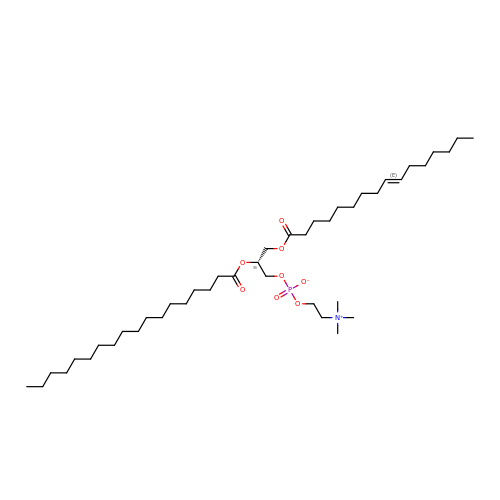[(2R)-3-[(E)-hexadec-9-enoyl]oxy-2-octadecanoyloxy-propyl] 2-(trimethylazaniumyl)ethyl phosphate | C42 H82 N O8 P | LJUDFFWSOQEQKW-NTUCYIKDSA-N(2S)-2-methyl-3-oxidanyl-propanoic acid 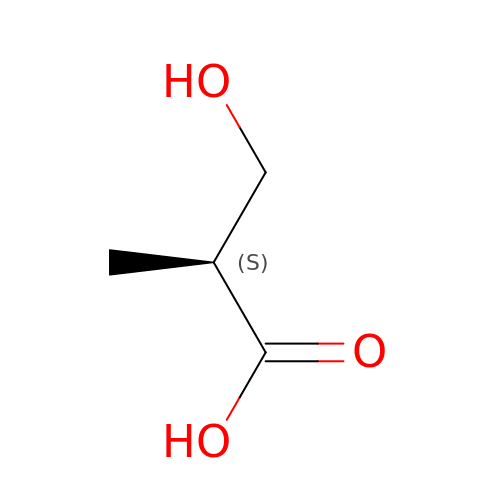| C4 H8 O3 | DBXBTMSZEOQQDU-VKHMYHEASA-N Contrasting with Enterobacteria, members of the dominant genus Bacteroides often encode several BtuB vitamin B12 outer membrane transporters together with a conserved array of surface-exposed B12-binding lipoproteins. Here we show that the BtuB transporters from Bacteroides thetaiotaomicron form stable, pedal bin-like complexes with surface-exposed BtuG lipoprotein lids, which bind B12 with high affinities. Closing of the BtuG lid following B12 capture causes destabilisation of the bound B12 by a conserved BtuB extracellular loop, causing translocation of the vitamin to BtuB and subsequent transport. We propose that TonB-dependent, lipoprotein-assisted small molecule uptake is a general feature of Bacteroides spp. that is important for the success of this genus in colonising the human gut.

However, BtuB3G3 incubated with excess CNCbl in the mild detergent Lauryl Maltose Neopentyl Glycol (LMNG) eluted as a single peak and had a pink colour after SEC, suggesting the presence of bound CNCbl. We determined the structure of this complex by cryo-EM. Data analysis produced maps of sufficient quality to build two slightly different models, named state 1 and state 2. Both states show density for a CNCbl molecule bound to BtuG3. A superposition of BtuG3-CNCbl onto BtuB3G3-CNCbl (state 1) has a Cα RMSD of ~0.6 Å, demonstrating that CNCbl binding to BtuG3 and BtuB3G3 is virtually identical. By contrast, in BtuB3G3-CNCbl (state 1), the EL8 loop has moved outwards to allow the vitamin to bind. The structural and functional data for the BtuB3G3-CNCbl complex, together with the comparison with the BtuG3-CNCbl and apo BtuB2G2 structures, suggest that the affinity of the CNCbl molecule for its BtuG3 binding site is lowered by the BtuB3 EL8 loop.

> MRRNILLVQFVGVLLLLPSIMSGQQHSSDNKNWAEKGIVIREVEILGKRPMKDIGVQQTRFDSLVLKENIALSMADILTFNSSIFVKSYGRATLSTVSFRGTSASHTQVTWNGMRINNPMLGMTDFSMIPSYFIDDASLLHGTSSVNMAGGGLGGLVKLSTVPAHQEGFGMQYVQGIGSFSTFDEFLQLKYGDKHWQISTRAVYQSSPNDYKYRNHDKKENIYDDKYNIIEQYYPIERNRSGAYKDLHILQEVYYNTGKGDRFGLNAWYTDSNRELALLTTDQGDLMDFENRQREHTLRSVLSWDHTRENWKVSARGGYVHTWLAYDYKRDLGNGIMATMTRSRSKVNTFYGQLDGEYFFSDKLLLTAGVSAHQHLVNSLDKDLNKDDNKNDKYGQGRKNDSIVYFDKGRIELSGNVSLKWQPVNRLGMSLVLRGEMFGTKWAPVIPAFFVDYVLSKRGNIMAKASITRNYRFPTLNDLYFLPGGNPALNNESGFTYETGLSFSVDKDNVYTLSGSASWFDQHINDWIIWLPTSKGFYSPVNLKKVHAYGVEVQADYAVAIDKAWKLGLNGTFAWTPSINEGEPTSKADQSVGKQLPYIPEYSATLSGRLTYRSWGLLYKWCYYSERYTMTSNAVSYTGHLPPYLMSNVTLEKGFSLRWADLSLKGTVNNLFDEEYLSVLSRPMPGINFEFFIGITPKWGKKKKGGGHHHHHH;> MKRILLSVLFIVFCLTAFVGCMKWDYGKMEPFRATGDGLFIMNEGNFQYGNATLSYYDPETKKVENEIFYRANAMKLGDVAQSMIVRDTIGWVVVNNSHVIFAISTNTFKEVGRITGLTSPRYIHFISDEKAYITQIWDYRIFIVNPKTYQITGYIECPDMTMETGSTEQMVQYGKYVYVNCWSYQNRILKIDTTTDKVVDQLTVGIQPTSLVMDKNFKMWTITDGGYKGSPYGYEEPSLYRIDAETFKIEKQFKFQLGDAPSEVQLNGAGDELYWINKDIWRMSVDEERVPVRPFLKYRDTKYYGLTVSPKNGDVYVADAIDYQQQGMIYRYTEDGELVDEFYVGIIPGAFCWK Inherited missense mutations in the myocilin (MYOC) gene, within its olfactomedin (OLF) domain, constitute the strongest genetic link to primary open-angle glaucoma via a toxic gain of function, and thus MYOC is an attractive precision-medicine target. Myocilin has no known function, and there is no glaucoma phenotype in Myoc knockout mice or in individuals with a homozygous N-terminal truncation mutation or hemizygous deletion of MYOC, but rare non-synonymous coding mutations lead to toxic intracellular sequestration of misfolded myocilin. However, not all mutations in MYOC cause glaucoma, and common variants are expected to be neutral polymorphisms. Among the common features associated with pathogenic myocilin misfolding, we demonstrate that a single metric, OLF thermal stability, can robustly segregate benign from early-onset disease variants.

At the outset of our study, five variants could be confidently predicted as benign polymorphisms: T293K, T353I, K398R, A445V and K500R. These mutations are all found on the protein surface and well documented in the literature. Three of these variants harbor conservative substitutions (Lys to Arg, Ala to Val). Assessment of spent media from cells expressing each of the 16 full-length myocilin variants revealed WT-like secretion for T256M, R296H, L303I, S313F, V329M, S331L, T353I, A445V, V449I and K500R. Analysis of the intracellular detergent-soluble fractions revealed E300K to be a statistical outlier among the variants, but T256M, S313F, N420Y, and A445V also presented decreased soluble protein levels compared to those of WT myocilin. Structural integrity was further confirmed by high-resolution crystal structures, which were solved for 11 OLF variants. No gross changes from WT OLF were detected for the structures of T293K, R296H, L303I, V329M, S331L, E352K, T353I, K398R, A445V, V449I or K500R, indicating that these mutations are accommodated within the native five-bladed β-propeller fold and do not perturb the dinuclear calcium-containing site.

> LKESPSGYLRSGEGDTGCGELVWVGEPLTLRTAETITGKYGVWMRDPKPTYPYTQETTWRIDTVGTDVRQVFEYDLISQFMQGYPSKVHILPRPLESTGAVVYSGSLYFQGAESRTVIRYELNTETVKAEKEIPGAGYHGQFPYSWGGYTDIDLAVDEAGLWVIYSTDEAKGAIVLSKLNPENLELEQTWETNIRKQSVANAFIICGTLYTVSSYTSVDATVNFAYDTGTGISKTLTIPFKNRYKYSSMIDYNPLEKKLFAWDNLNMVTYDIKLSKM> GPLGSGIQMENSWTISKEYHIDEEVGFALPNPQENLPDFYNDWMFIAKHLPDLIE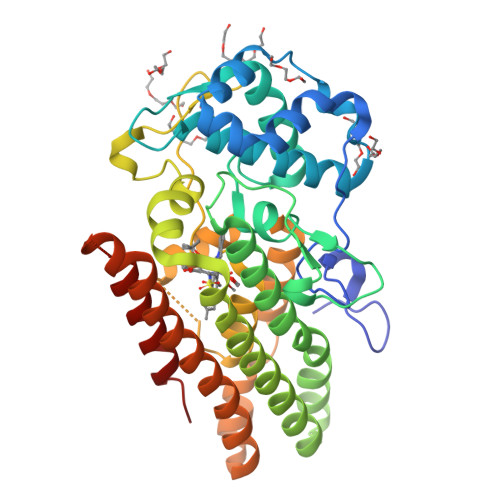SGQLRERVEKLNMLSIDHLTDHKSQRLARLVLGCITMAYVWGKGHGDVRKVLPRNIAVPYCQLSKKLELPPILVYADCVLANWKKKDPNKPLTYENMDVLFSFRDGDCSKGFFLVSLLVEIAAASAIKVIPTVFKAMQMQERDTLLKALLEIASCLEKALQVFHQIHDHVNPKAFFSVLRIYLSGWKGNPQLSDGLVYEGFWEDPKEFAGGSAGQSSVFQCFDVLLGIQQTAGGGHAAQFLQDMRRYMPPAHRNFLCSLESNPSVREFVLSKGDAGLREAYDACVKALVSLRSYHLQIVTKYILIPASQQPKENKTSEDPSKLEAKGTGGTDLMNFLKTVRSTTEKSLL>MASQVTDMRSNSQGLSLTDSVYERLLSERIIFLGSEVNDE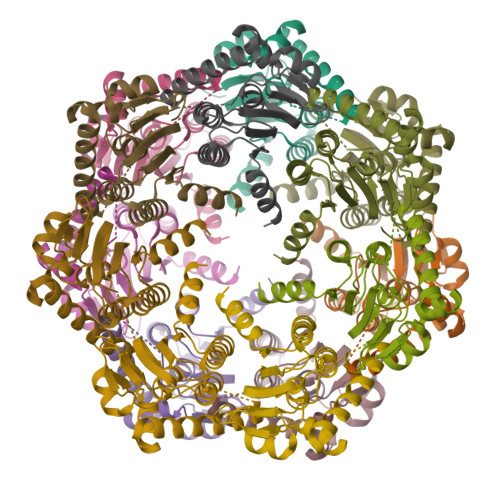IANRLCAQILLLAAEDASKDISLYINSPGGSISAGMAIYDTMVLAPCDIATYAMGMAASMGEFLLAAGTKGKRYALPHARILMHQPLGGVTGSAADIAIQAEQFAVIKKEMFRLNAEFTGQPIERIEADSDRDRWFTAAEALEYGFVDHIITRAHVNGEAQGHHHH[14x]> GHMQETQAVEAGEKTVEQFVQALNKGDYNKAAEMTSKKAANKSALSEKEILDKYQNIYGAADVKGLQISNLKVDKKDDSTYSFSYKAKMNTSLGELKDLSYKGTLDRNDGQTTINWQPNLVFPEMEGNDKVSLTTQEAARGNIIDRNGEPLATTGKLKQLGVVPSKLGDGGEKTANIKAIASSFDLTE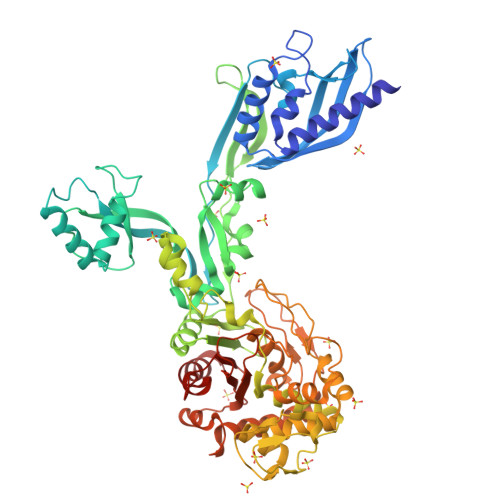DAINQAISQSWVQPDYFVPLKIIDGATPELPAGATIQEVDGRYYPLGEAAAQLIGYVGDITAEDIDKNPELSSNGKIGRSGLEMAFDKDLRGTTGGKLSITDADGVEKKVLIEHEVQNGKDIKLTIDAKAQKTAFDSLGGKAGSTVATTPKTGDLLALASSPSYDPNKMTNGISQEDYKAYEENPEQPFISRFATGYAPGSTFKMITAAIGLDNGTIDPNEVLTINGLKWQKDSSWGSYQVTRVSDVSQVDLKTALIYSDNIYTAQETLKMGEKKFRTGLDKFIFGEDLDLPISMNPAQISNEDSFNSDILLADTGYGQGELLINPIQQAAMYSVFANNGTLVYPKLIADKETKDKKNVIGETAVQTIVPDLREVVQDVNGTAHSLSALGIPLAAKTGTAEIPAPAPAPGKENSFLFAFNPDNQGYMMVSMLENKEDDDSATKRASELLQYLNQNYQ> MPKPINVRVTTMDAE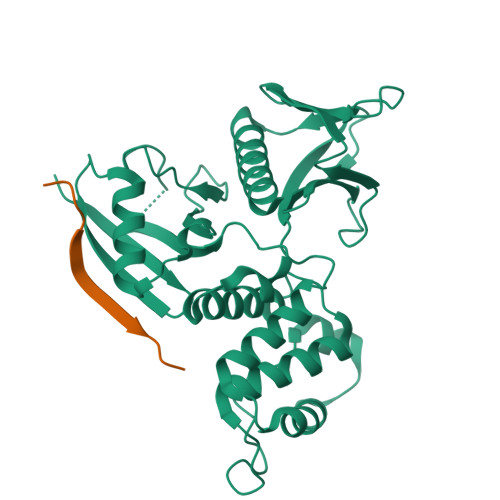LEFAIQPNTTGKQLFDQVVKTIGLREVWYFGLHYVDNKGFPTWLKLDKKVSAQEVRKENPLQFKFRAKFYPEDVAEELIQDITQKLFFLQVKEGILSDEIYCPPETAVLLGSYAVQAKFGDYNKEVHKSGYLSSERLIPQRVMDQHKLTRDQWEDRIQVWHAEHRGMLKDNAMLEYLKIAQDLEMYGINYFEIKNKKGTDLWLGVDALGLNIYEKDDKLTPKIGFPWSEIRNISFNDKKFVIKPIDKKAPDFVFYAPRLRINKRILQLCMGNHELYMRRRK;> DSEPVLKGVKLHYT>GSAKDPMKVTVIGCYGGFPAANEATSGYLFQSGDYSLLVDCGSAVLSKLFGYVPAEKLDAVILSHYHHDHIADIGPLQFAKQVGSFLGKGEHTLPIYGHDADIEQFQKLTYKTHTKGIAFQPDQPLTAGPFTITFLKTIHPVTCYAMRITDGSHTVVYTADSSYQDSFIPFSENADLLISECNFYADQDGTSAGHMNSLEAGRIAKEAGAGELLLTHLPHFGVHDNLRKEAKTVF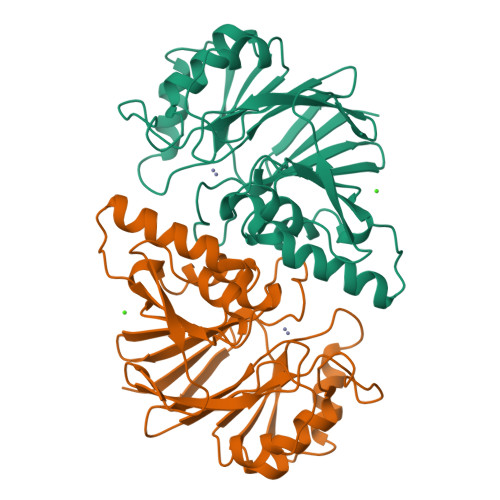SGEVNIAKSGFVWEG[4x]3-(3-methyl-4-oxo-3,4-dihydroquinazolin-2-yl)propanoic acid | C12 H12 N2 O3 | 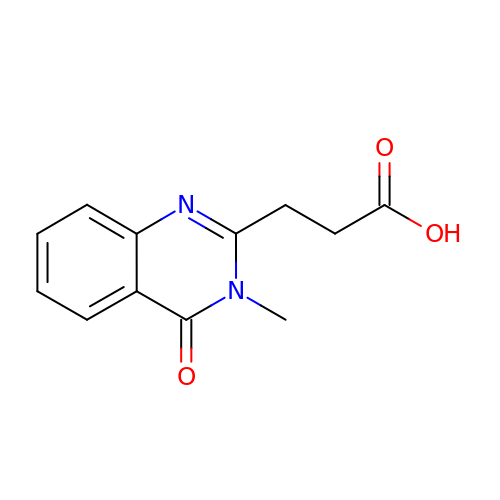UXGWMRNLTMHSST-UHFFFAOYSA-N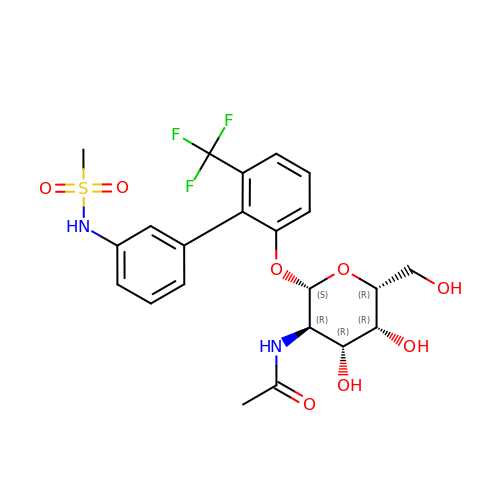N-[2'-{[2-(acetylamino)-2-deoxy-beta-D-galactopyranosyl]oxy}-6'-(trifluoromethyl)[1,1'-biphenyl]-3-yl]methanesulfonamide | C22 H25 F3 N2 O8 S | RPOJFLNPFLSKOB-QNDFHXLGSA-N>MNTVSPAKKKVIIIGAGIAGLKAASTLHQNGIQDCLVLEARDRVGGRLQTVTGYQGRKYDIGASWHHDTLTNPLFLEEAQLSLNDGRTRFVFDDDNFIYIDEE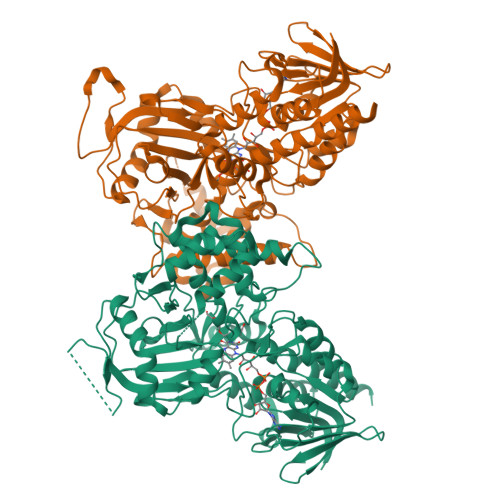RGRVDHDKELLLEIVDNEMSKFAELEFHQHLGVSDCSFFQLVMKYLLQRRQFLTNDQIRYLPQLCRYLELWHGLDWKLLSAKDTYFGHQGRAAFALNYDSVVQRIAQSFPQNWLKLSCEVKSITREPSKNVTVNCEDGTVYNADYVIITVPQSVLNLSVQPEKNLRGRIEFQPPLKPVIQDAFDKIHFGALGKVIFEFEECCWSNESSKIVTLANSTNEFVEIVRNAENLDELDSMLEREDSQKHTSVTCWSQPLFFVNLSKSTGVASFMMLMQAPLTNHIESIREDKERLFSFFQPVLNKIMKCLDSEDVIDGMRPIENIANANKPVLRNIIVSNWTRDPYSRGAYSACFPGDDPVDMVVAMSNGQDSRIRFAGEHTIMDGAGCAYGAWESGRREATRISDLLKLEHHHHHH[4x]> GPDLVQKLKVLRHELSLQQPQAGHCRIEVSREEIFEESYRQIMKMRPKDLKKRLMVKFRGEEGLDYGGVAREWLYLLCHEMLNPYYGLFQYSTDNIYMLQINPDSSINPDHLSYFHFVGRIMGLAVFHGHYINGGFTVPFYKQLLGKPIQLSDLESVDPELHKSLVWILENDITPVLDHTFCVEHNAFGRILQHELKPNGRNVPVTEENKKEYVRLYVNWRFMRGIEAQFLALQKGFNELIPQHLLKPFDQKELELIIGGLDKIDLNDWKSNTRLKHCVA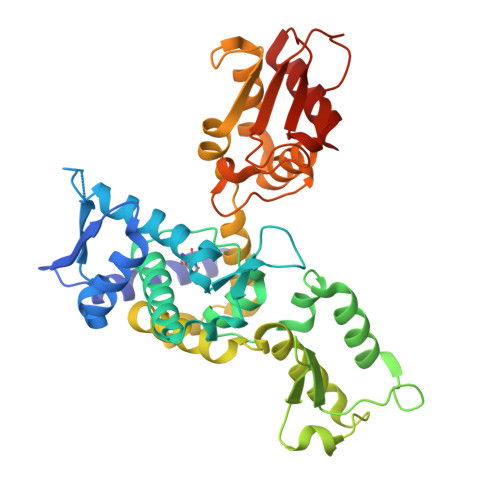DSNIVRWFWQAVETFDEERRARLLQFVTGSTRVPLQGFKALQGSTGAAGPRLFTIHLIDANTDNLPKAHTCFNRIDIPPYESYEKLYEKLLTAVEET>[4x]HMRLIEDICLPRWGCLWEDDDKLPNIVILATGGTIAGSAATGTQTTGYKIGALGVDTLINAVPEVKKLANVKGEQFSNMASQNMTGDVVLKLSQRVNELLARDDVDGVVITHGTDTVEESAYFLHLTVK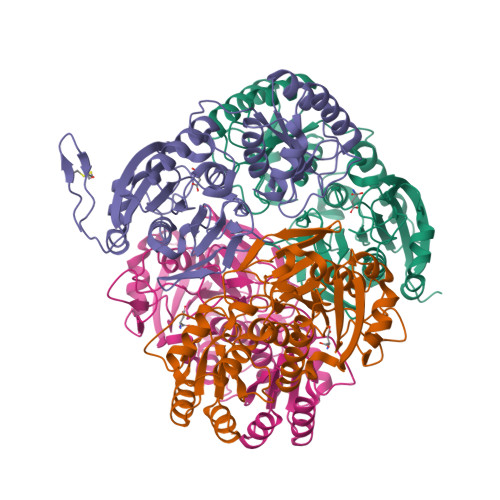SDKPVVFVAAMRPATAISADGPMNLLEAVRVAGDKQSRGRGVMVVLNDRIGSARYITKTNASTLDTFKANEEGYLGVIIGNRIYYQNRIDKLHTTRSVFDVRGLTSLPKVDILYGYQDDPEYLYDAAIQHGVKGIVYAGMGAGQVSVRGIAGMRKAMEKGVVVIRSTRTGNGIVPPDEELPGLVSDSLNPAHARILLMLALTRTSDPKVIQEYFHTY6-amino-2-[(2-phenylethyl)amino]-1,7-dihydro-8H-imidazo[4,5-g]quinazolin-8-one 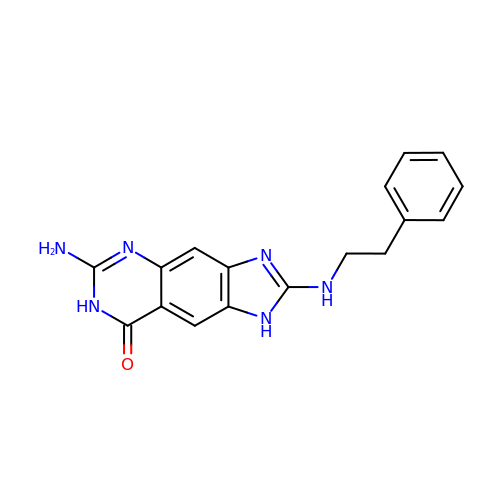| C17 H16 N6 O | IGMWKNNADHYQOB-UHFFFAOYSA-N> GVTGPPDPQVRCPSVIEFGKYEIHTWY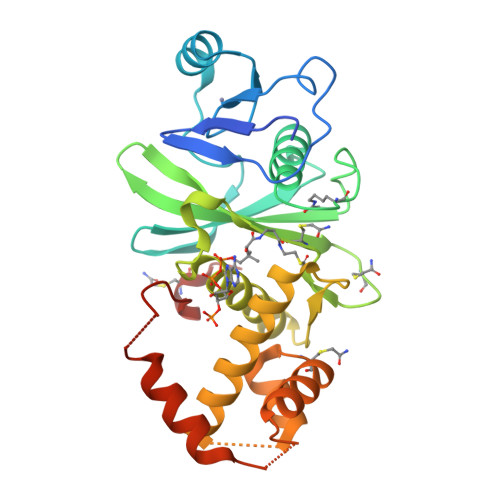SSPYPQEYSRLPKLYLCEFCLKYMKSRTILQQHMKKCGWFHPPANEIYRKNNISVFEVDGNVSTIYCQNLCLLAKLFLDHKTLYYDVEPFLFYVLTQNDVKGCHLVGYFSKEKHCQQKYNVSCIMILPQYQRKGYGRFLIDFSYLLSKREGQAGSPEKPLSDLGRLSYMAYWKSVILECLYHQNDKQISIKKLSKLTGICPQDITSTLHHLRMLDFRSDQFVIIRREKLIQDHMAKLQLNLRPVDVDPECLRWTPVI>GPLGSSELDKIQSELLNYTDDTLPAMENVDAIKDKMSYWRRTQFAVLPMKDEAQIRQTIERNNRVQAEINDSLVAYGKTVWPGEEEQTFKRLMGNWNAYTAVTDQFNQTLLTQGADDAYPILANSLSTFEALESDFTLLIGILHQAMDSNKVQI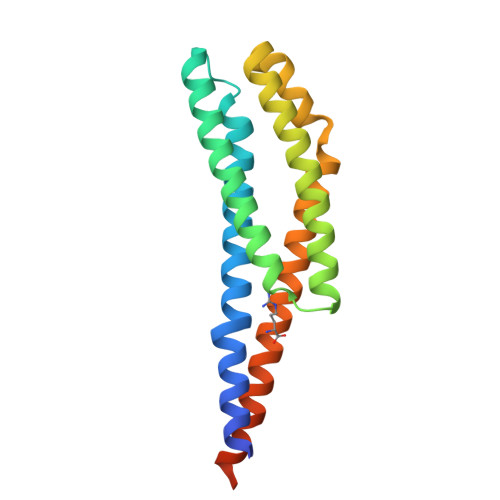LSSVKTLNSTSEFPGRLERPHRD[2x]> GSHMSRPPSR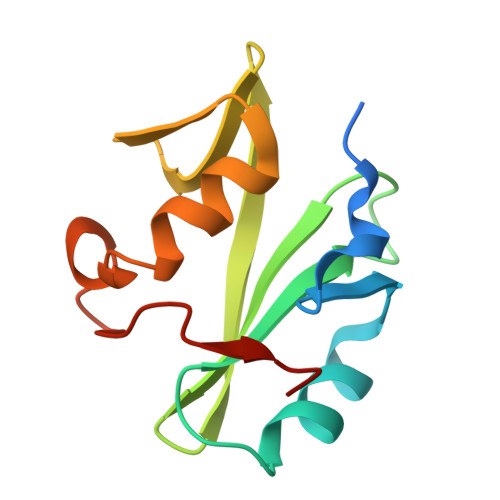EIDYTAYPWFAGNMERQQTDNLLKSHASGTYLIRERPAEAERFAISIKFNDEVKHIKVVEKDNWIHITEAKKFDSLLELVEYYQCHSLKESFKQLDTTLKYPYKSRE>MSKLAIIAGDGIGPEVTAEAVKVLDAVVPGVQKTSYDLGARRFHATGEVLPDSVVAELRNHDAILLGAIGDPSVPSGVLERGLLLRLRFELDHHINLRPARLYPGVASPLSGNPGIDFVVVREGTEGPYTGNGGAIRVGTPNEVATEVSVNTAFGVRRVVADAFERARRRRKHLTLVHKTNVLTFAGGLWLRTVDEVGECYPDVEVAYQHVDAATIHMITDPGRFDVIVTDNLFGDIITDLAAAVCGGIGLAASGNIDATRANPSMFEPVHGSAPDIAGQGIADPTAAIMSVALLLSHLGEHDAAARVDRAVEAHLATRGSERLATSDVGE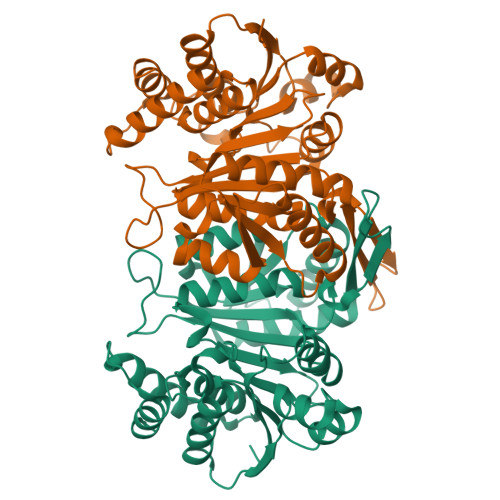RIAAAL[4x]(2R,3R)-6-methyl-2,3-bis(oxidanyl)heptanoic 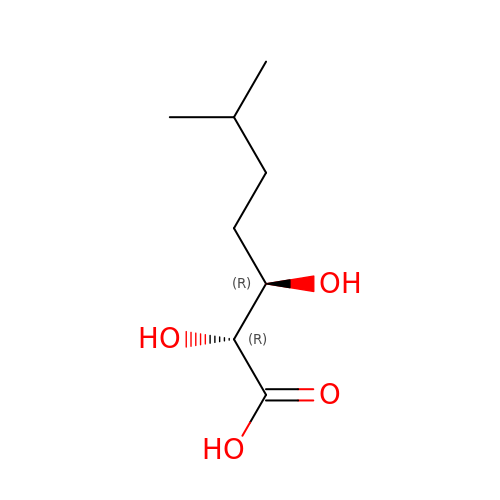acid | C8 H16 O4 | GGZLDTFSYRKUEP-RNFRBKRXSA-N> NRIITEYILIDANNYHFKSWIECFPDCKVNLKLLLFRPEWFDFFKYVESKTYFPQ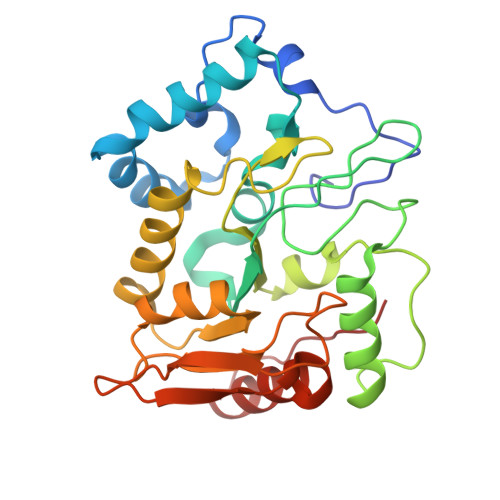LESKLSSYLEKRQRIVPYPELLFNTMNVLPPGKIKVVILGQDPYPGSCISGVPYAMGCSFSVPLNCPVPKSLANIYTNLIKFNHMRKAPKHGCLASWILQGTFMINSAFTTVLNESGVHARTWESFTADLIDYLTDNYDDLIFVAWGAHAHKLCQRVDPKKHYIITSSHPSPLSVSNTMTSMSYGPNPKKVTYPSFNSVDHFGKINEHLKSRNKKPIFWDL N-{3-[(2E,4R)-2-imino-1-methyl-5-oxo-4-phenylimidazolidin-4-yl]phenyl}furan-2-carboxamide 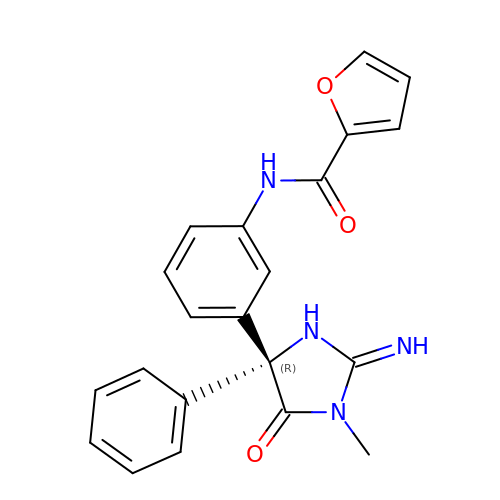| C21 H18 N4 O3 | SOHROZVXKZYZIE-OAQYLSRUSA-N>[2x]GAILAARIAVSNLHKETKKVFSDVMEDLYNYINPHNGKHSPMVAKSTLDIVLANKDRLNSAIIYDRDFSYNY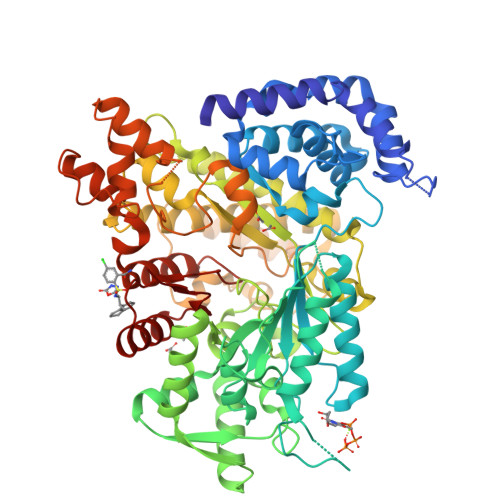FGFKTLERSYLLKINGKVAERPQHMLMRVSVGIHKEDIDAAIETYNLLSERWFTHASPTLFNAGTNRPQLSSCFLLSMKDDSIEGIYDTLKQCALISKSAGGIGVAVSCIRATGSYIAGTNGNSNGLVPMLRVYNNTARYVDQGGNKRPGAFAIYLEPWHLDIFEFLDLKKNTGKEEQRARDLFFALWIPDLFMKRVETNQDWSLMCPNECPGLDEVWGEEFEKLYASYEKQGRVRKVVKAQQLWYAIIESQTETGTPYMLYKDSCNRKSNQQNLGTIKCSNLCTEIVEYTSKDEVAVCNLASLALNMYVTSEHTYDFKKLAEVTKVVVRNLNKIIDINYYPVPEACLSNKRHRPIGIGVQGLADAFILMRYPFESAEAQLLNKQIFETIYYGALEASCDLAKEQGPYETYEGSPVSKGILQYDMWNVTPTDLWDWKVLKEKIAKYGIRNSLLIAPMPTASTAQILGNNESIEPYTSNIYTRRVLSGEFQIVNPHLLKDLTERGLWHEEMKNQIIACNGSIQSIPEIPDDLKQLYKTVWEISQKTVLKMAAERGAFIDQSQSLNIHIAEPNYGKLTSMHFYGWKQGLKTGMYYLRTR>GAFLDKPKMEKHNAQGQGNGLRYGLSSMQGWRVEMEDAHTAVIGLPSG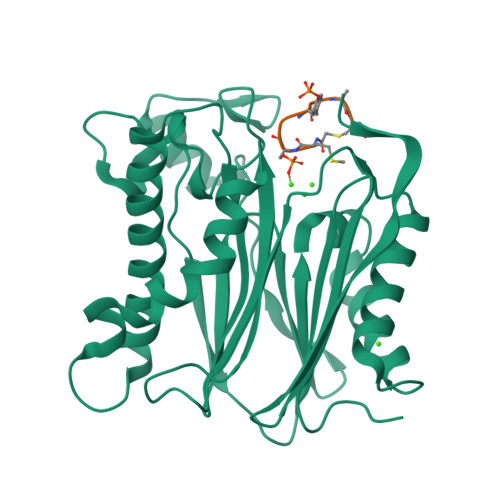LESWSFFAVYDGHAGSQVAKYCCEHLLDHITNNQDFKGSAGAPSVENVKNGIRTGFLEIDEHMRVMSEKKHGADRSGSTAVGVLISPQHTYFINCGESRGLLCRNRKVHFFTQDHKPSNPLEKERIQNAGGSVMIQRVNGSLAVSRALGDFDYKCVHGKGPTEQLVSPEPEVHDIERSEEDDQFIILACDGIWDVMGNEELCDFVRSRLEVTDDLEKVCNEVVDTCLYKGSRDNMSVILICFPNAPKV[3x];>[3x]MSIYVAX> AYPMPNPFPPFRIAGNLYYVGTDDLASYLIVTPRGNILINSDLEANVPMIKASIKKLGFKFSDTKILLISHAHFDHAAGSELIKQQTKAKYMVMDEDVSVILSGGKSDFHYANDSSTYFTQSTV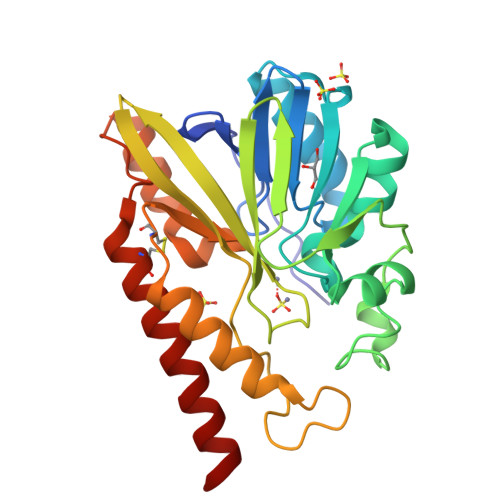DKVLHDGERVELGGTVLTAHLTPGHTRGCTTWTMKLKDHGKQYQAVIIGSIGVNPGYKLVDNITYPKIAEDYKHSIKVLESMRCDIFLGSHAGMFDLKNKYVLLSKGQNNPFVDPTGCKNYIEQKANDFYTELKKQETG> GPELVMRRGEIWQVDLDPARGSEANNQRPAVVVSNDRANATATRLGRGVITVVPVTSNIAKVYPF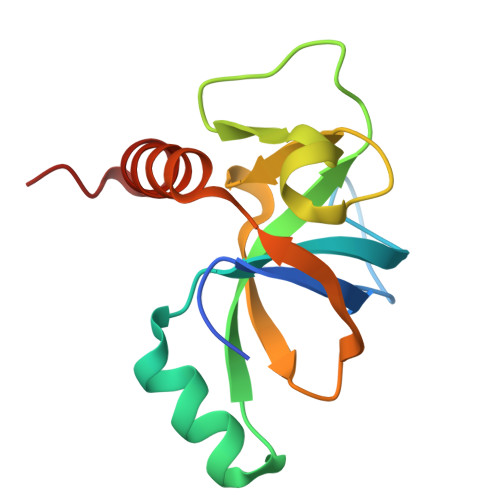QVLLSATTTGLQVDCKAQAEQIRSIATERLLRPIGRVSAAELAQLDEALKLHLDLWS> MFSKAPRPASCKPLSSKEVISIQKGATDLGKALFYAIKHQDYKHASELVALGAPIERCYEVEKDVYRTTCSLLVGMICTARIAKGHREISYRIPDRILDTFIQLGVDLRCHCSNKFEHRCPLFVALKILNVQNEQEL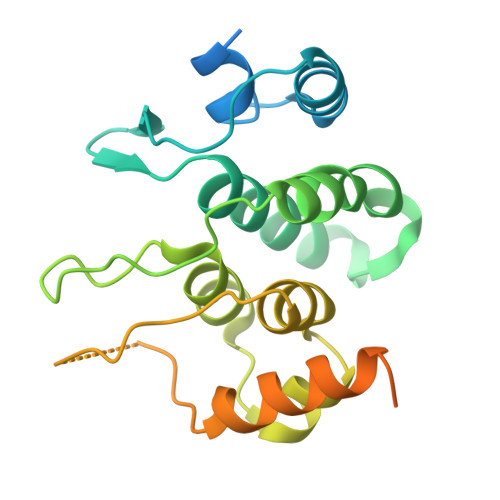FKDKNQIVQKLIINGATIKNHIQPHKTFHNIPHFDIEGIRSYLISKSQLASVKKSGSLQTATSNYHDNCKNPLPYKHNSEFSKTGYNFTFQYK> MHHHHHHENLYFQGTVVTTESGLKYEDLTEGSGAEARAGQTVSVHYTGWLTDGQKFDSSKDRNDPFAFVLGGGMVIKGWDEGVQGMKVGGVRRLTIPPQLGYGARGAGGVIPPNATLVFEVELLDV

Macrophage infectivity potentiator (MIP) proteins are key microbial virulence factors that facilitate host cell infection, intracellular pathogen replication, and dissemination. They are found in a variety of pathogens of both bacterial and eukaryotic origin, including Burkholderia pseudomallei, the causative agent of melioidosis, Legionella pneumophila, leading to Legionnaires’ disease, and the protozoan parasites Trypanosoma cruzi and Leishmania subspecies. All MIP proteins share a peptidyl-prolyl-cis–trans-isomerase (PPIase) domain resembling the FK506 binding protein domains of human FKBPs. All MIP and FKBP proteins share a general domain topology in their core PPIase domain with an amphipathic five-stranded β-sheet wrapping around a short α-helix, thereby forming a hydrophobic active site32. Inhibition of secreted MIP proteins diminishes macrophage invasion and leads to the reduction of overall pathogen load and virulence, as shown for L. pneumophila and B. pseudomallei, respectively.

Here, we determined the crystal structures of B. pseudomallei MIP (BpMIP), which contains only the core PPIase domain and T. cruzi MIP (TcMIP), which features the PPIase domain and a free-standing α-helix (“stalk”), in complex with fluorinated pipecolic acid inhibitors. In all cases, we found that the inhibitor molecules bound within the expected FKBP-like domain cleft that forms the MIP active site. In the PPIase assay, clear inhibitory activity of both NJS224 and NJS227 was observed against every MIP. These compounds were originally developed to inhibit BpMIP and thus showed strong activity against this protein with Ki values of 21 ± 2 and 90 ± 10 nM, respectively. Comparing the crystal structures of TcMIP and BpMIP with NJS227, the inhibitor adopts a highly similar binding stance and the respective protein side chains align well (RMSD = 0.58 Å). The fluorobenzyl group attached to the sulfoxyl group, i.e., the group present in either inhibitor, is nestled into a hydrophobic pocket formed by F43 in β-strand 3a and V97/I98 in the loop between β4 and β5 in BpMIP and the corresponding residues F73 and M125/I126 in TcMIP. This leads to near perfectly superimposable fluorobenzyl moieties across all crystallized inhibitor complexes. In the crystal structure of BpMIP in complex with NJS227, the sulfoxyl moiety oxygens are 3.5 and 3.3 Å apart from the oxygen atoms of the side chains of D434 in β3a and Y88 in the β4/β5 loop. In the crystal structures, the inhibitor’s piperidine ring rests within a hydrophobic cage formed by conserved aromatic residues (Y33/Y63, F53/F85, and W66/W94 in BpMIP and TcMIP, respectively). In BpMIP and TcMIP, hydrophobic residues in this region (V62/I63 in BpMIP and V90/I91 in TcMIP) interact with the inhibitor pyridine group.> EAEASICSEPKKVG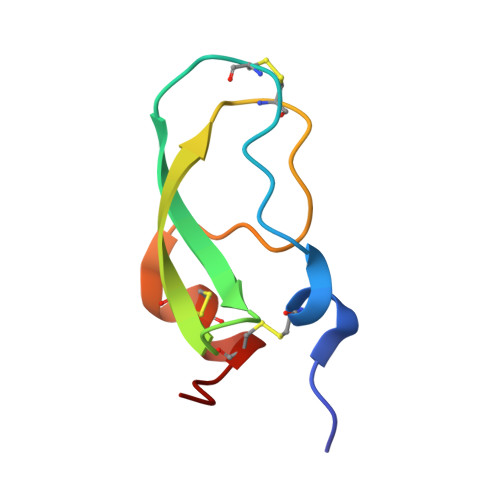RCKGYFPRFYFDSETGKCTPFIYGGCGGNGNNFETLHQCRAICRALG>QANLMRLKSDLFNRSPMYPGPTKDDPLTVTLGFTLQDIVKVDSSTNEVDLVYYEQQRWKLNSLMWDPNEYGNITDFRTSAADIWTPDITAYSSTRPVQVLSPQIAVVTHDGSVMFIPAQRLSFMCDPTGVDSEEGVTCAVKFGSWVYSGFEIDLKTDTDQVDLSSYYASSKYEILSATQTRQVQHYSCCPEPYIDVNLVVKFRERRAGNGFFRNLFD[5x]

Cys-loop receptors are a class of pentameric ligand-gated ion channels that are activated by specific neurotransmitters, including acetylcholine (ACh), serotonin (5-HT), glycine (Gly), and γ-aminobutyric acid (GABA). Recently, Gao et al. characterized an extensive set of mutants in acetylcholine binding protein (AChBP), a structural and functional homolog of the extracellular domain of the nAChR. Using X-ray crystallography we solved 3-dimensional structures of strychnine or d-tubocurarine in complex with ACh binding protein (AChBP), a well-recognized structural homolog of the nicotinic ACh receptor. Our results demonstrate that AChBP binds strychnine and d-TC with high affinity and serves as an appropriate model for mapping the binding site topography in different CLRs, including the GlyR, nAChR, and 5-HT3R.

The affinity of strychnine for Ac-AChBP (Ki = 38.0±3.3 nM) is more than 100-fold higher than for α7 nAChR (Ki = 4,854±133 nM) and is actually close to the high affinity of strychnine reported for the α1 GlyR (Ki = 16±2 nM). The crystal structure of Aplysia AChBP in complex with strychnine contains 1 pentamer in the asymmetric unit. Inspection of simple difference electron density unambiguously revealed the ligand orientation in all five binding sites of the pentamer. Remarkably, one of the two C loops involved in forming a crystal contact is in a more extended conformation and reveals electron density for a second strychnine molecule in the same binding site. The first strychnine molecule, which contacts the (+) face, is pivoted by 48° around the N-atom relative to the strychnine molecule in all other four binding sites (single occupancy in yellow and double occupancy in magenta). The second strychnine molecule, which contacts the (−) face, is stacked onto the first molecule in a mirrored upside-down orientation and both molecules are separated by a distance of 3.6 Å. In the binding site with double occupancy, the tip of loop C is displaced outward by a distance of 5.6 Å relative to the binding sites with single occupancy. First, strychnine forms contacts with the following residues on the (+) face: Y91, S144, W145, C188, C189, Y193 and (−) face: Y53, Q55, M114, I116, D162, S165. Three additional contacts are formed in the binding site with double ligand occupancy, namely Y186 on the (+) face and T34, R57 on the (−) face. Because the C-loop interacting with 2 strychnine molecules also interfaces with a C-loop from a neighboring pentamer the double strychnine occupancy might be the result of a crystal contact.> GAMGSTVGLTALKVSGETLSEPMRPGVIRFGLTPVFLSNDLEVLDELQAYLTQAVGQEVQLITQRTYQEVTALLVSGNLEAAWICGYPFMKFRDELDLVATPLWRGKPVYQSYLIVGRDRDIAGFEDCQGDIHAFSDPDSNSGYLVTKTYLAERGVSEEGFFRKSFFTYGHRNVIRAVASGLADSGSVDGYVWEVMKTTEPELVAKTRVLVKSGWHGFPPVAAAAGQRKSQAVARIRSALLDMNQEVLGRSVLTRLQLDGFVETTAESYDSIAANMERVRRLG

The regulatory cluster consists of three genes, aioX, aioS and aioR, which encode a periplasmic-binding protein (PBP), a sensor histidine kinase and a response regulator, respectively. Arsenite-bound AioX is thought to act as a ligand for AioS, the sensor histidine kinase that upon auto-phosphorylation, phosphorylates AioR, the response regulator, which binds to a conserved sequence upstream of a RpoN promoter. AioX exhibits a typical bilobed structure of the PBP type II class. In this class of proteins, the ligand-binding pocket is located in the space between the two domains.

In the initial single-wavelength anomalous diffraction (SAD) electron density maps generated from the crystals of Se-Met labelled protein there was an unaccounted electron density in the putative ligand-binding region near residue Cys106. The electron density was consistent with the presence of a phosphate ion, from the crystallisation conditions, and its location would suggest that Cys106 might be involved in binding arsenite. The crystal structure of the phosphate-bound AioX was used to solve the structures of the apo and arsenite-bound forms of the protein by molecular replacement. On the other hand, a phosphate ion found in the binding site of AioX formed AioX-specific hydrogen bonds with Asp210 and Cys106, which in PhnD correspond to Asn175 and Gly65, respectively. The presence of a phosphate ion in the binding site of AioX leads to the hypothesis that the phosphate ion mimics arsenite binding. A comparison of the X-ray structures however, indicates that while AioX can bind phosphate, the resulting structure does not stabilize the 53–61 loop conformation seen in the arsenite-bound form. Furthermore, even though the structure is similar to the arsenite-bound form, with the main conformation of Tyr88 akin to that of the arsenite-AioX, electron density for residues 53–61 are ambiguous and due to the disorder, we were unable to confidently build a model for residues 55–57. Within region 55–57 the structure had more similarity to the apo rather than the arsenite-bound form of AioX. As we were unable to detect any binding interaction, based on the conditions used in the ITC we estimate that the Kd for phosphate would have to be greater than 2 mM (data not shown). As AioX and ArxX did not bind phosphate in conditions tested in ITC, we conclude that AioX and ArxX do not bind phosphate under biologically relevant conditions.> MTMEQFLTSLDMIRSGCAPKFKL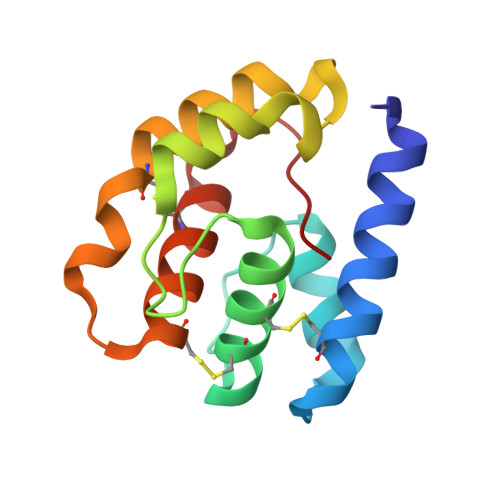KTEDLDRLRVGDFNFPPSQDLMCYTKCVSLMAGTVNKKGEFNAPKALAQLPHLVPPEMMEMSRKSVEACRDTHKQFKESCERVYQTAKCFSENADGQFMWP>[8x]MGPEEILERAKESLERAREASERGDEEEFRKAAEKALELAKRLVEQAKKEGDPELVLEAARVALWVAELAAKNGDKEVFKKAAESALEVAKRLVEVASKEGDPDLVAWAALV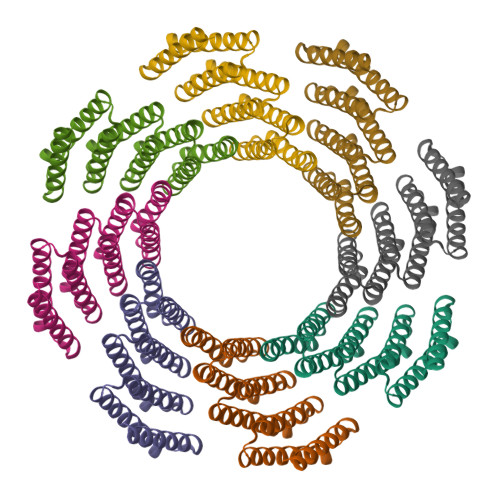ALWVAFLAFLNGDKEVFKKAAESALEVAKALMEVAMKVGAPWLVELAIAVARAVWLLAELFGDEEVRRRAEAFEIILRIAAIAVKAWLGGGGSLEHHHHHH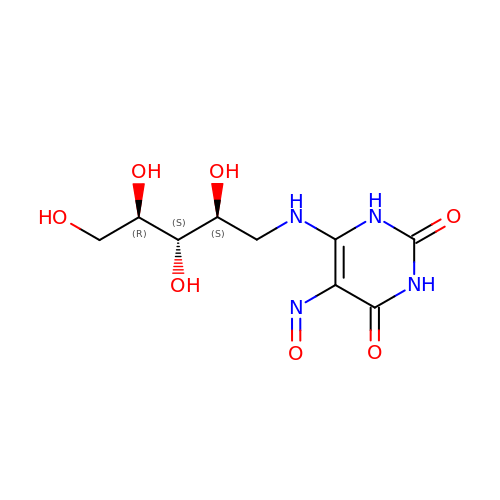5-NITROSO-6-RIBITYL-AMINO-2,4(1H,3H)-PYRIMIDINEDIONE | C9 H14 N4 O7 | YMWIHKCBRFEJMH-RPDRRWSUSA-N>MNNSFLDKLIETKELKNSLYNVLKHNFLYHANKIAGSTFTTEALALLLDKNVVTGRHTLDDVQETVNSSYVFDTVIDSLKEKITHNFLRNLHSSLIFNTTLHSRGMAGIYKTIPNMILGTDVSIAQPFEVEPKLDELIEWYYSQSEVSIKVIAEFHYRFELIHPFQDGNGRIGRFVM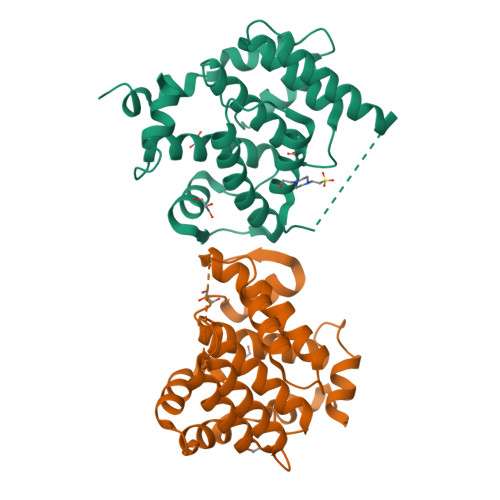LKQMLENNLPIKIVSWDSEDLYRNSLNSCSLGNYVPLIEYLSSLEDFREVYKMLWKLE[2x]Crystal structures of the two sub-structures of U1 snRNP. molecular details of 5′SS recognition by U1 snRNP. intricate network of interactions between the components of U1 snRNP. insights into the molecular mechanism of 5′SS selection.

60–216 of U1-70k via Gly–Ser linker. stem-loop I and U1-70k in detail, illustrating a new mode of RRM-RNA interaction. (A) Interaction of stem-loop I with U1-70k RRM. (A) C33 and G34 embraced by U1-70k loop 3. and A32 stack onto Phe106 and Phe148 residues of the beta sheet. loop is closed by a trans WC/Hoogsteen base pair formed between A29 and A36. strand the bases A35, A36, G37 and G38 continuously stack. along with A29 and Arg190, continues the helical stacking of the stem. (B) Interaction of stem-loop II with U1-A RRM. detailed RNA-protein contacts between U1-A RRM and stem-loop II.

> GVPETRPNHTIYINNLNEKIKKDELKKSLYAIFSQFGQILDILVSRSLKMRGQAFVIFKEVSSATNALRSMQGFPFYDKPMRIQYAKTDSDIIAKMKGTFVERDRKREKRGSGSGSGSGSGSGAETREERMERKRREKIERRQQEVETELKMWDPHNDPNAQGDAFKTLFVARVNYDTTESKLRREFEVYGPIKRIHMVYSKRSGKPRGYAFIEYEHERDMHSAYKHADGKKIDGRRVLVDVERGRTVKGWRPRRLGGGLGGTRRGGADVNIRHSGRDD>[4x]MDYKDDDDKMQPDMSLNVIKMKSSDFLESAELDSGGFGKVSLAFHRTQGLMIMKTVYKGPNCIEHNEALLEEAKMMNRLRHSRVVKLLGVIIEEGKYSLVMEYME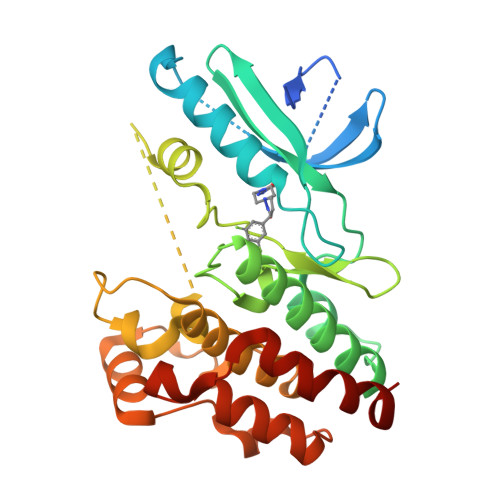KGNLMHVLKAEMSTPLSVKGRIILEIIEGMAYLHGKGVIHKDLKPENILVDNDFHIKIADLGLASFKMWSKLNNEEHNELREVDGTAKKNGGTLYYMAPEHLNDVNAKPTEKSDVYSFAVVLWAIFANKEPYENAIAEQQLIMAIKSGNRPDVDDITEYCPREIISLMKLCWEANPEARPTFPGIEEKFRPFYLSQLE>[4x]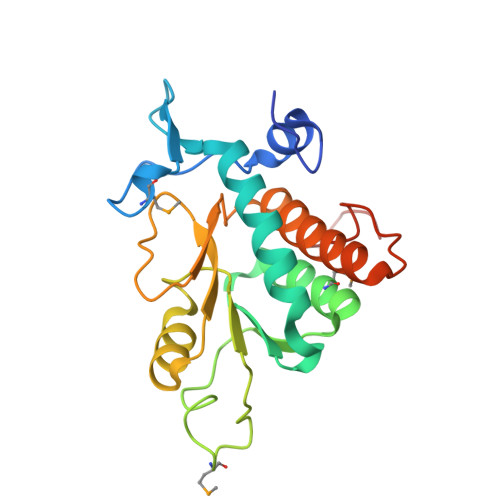MSLEKEYEYLVPPDDYLAAGVHIGTQIKTGDMKKFIFKVRQDGLYVLDIRKLDERIRVAAKFLSRYEPSKILLVAARQYAHKPVQMFSKVVGSDYIVGRFIPGTLTNPMLSEYREPEVVFVNDPAIDKQAVSEATAVGIPVVALCDSNNSSADVDLVIPTNNKGRRALAIVYWLLAREIAKIRGQDFTYSIEDFEAELEGGSHHHHHH> CGCTATAATGCG

The Pribnow box consensus sequence is the sequence 5′-TATAAT-3′ of six nucleotides that is an essential part of a promoter site of DNA – located at the −10 position upstream of the bacterial transcription start site for transcription to occur in prokaryotes. Non-complementary base pairs or mismatches can occur due to a range of factors such as replication errors, misincorporations and cytosine methylation, at a frequency of 1 per 109–1010 base pairs per cell division, and these alter the natural interaction between base pairs. The crystal structure presented here shows bending of the DNA at the mismatch point after metalloinsertion by the ruthenium complexes. The metal complex interacts with the DNA via the major groove, where specific interactions between the adenines of the DNA and the phen ligands of the complex are formed.

The overall effect of the kinking is to open up the major groove and compress the minor groove. A central twofold rotation axis relates the two halves of the assembly. At each end there are three CG base pairs, with the central TATAAT sequence binding the two Λ-complexes and showing a modified base pairing pattern to accommodate the mismatches. The T4 base pairs with A8 on the opposite strand, so that T9 is flipped out. This shift allows T6 to pair with A7 on the opposite strand. As the two phen moieties are approximately orthogonal, constrained by the rigid octahedral geometry of the metal centre, the extremely flexible DNA strand kinks such that the adenine base planes make an 80° dihedral angle, similar to the 86.5° angle between the phen ligands. The strength and specificity of the interaction is enhanced by the formation of a hydrogen bond between one imino H of the phi ligand and the N3 nitrogen of A7, with an N–N distance of 3.0 Å. The single complex lies on the twofold rotation axis, with the phi ligands of the Λ-complex stacking on the phi ligand of the Δ-enantiomer, and is enclosed by the kinked and metal bound duplex.> CCGAUGGUAGUG;> GCGAGAGUAG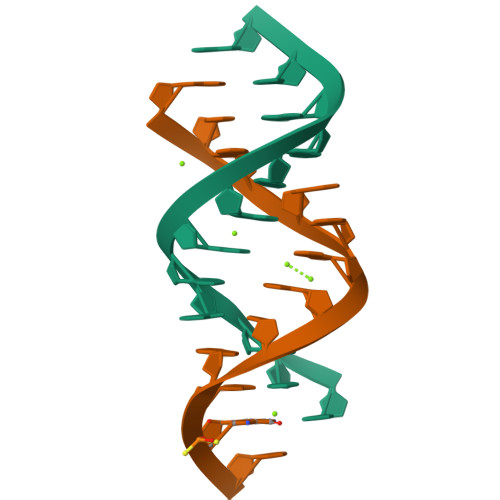GC>GMKGENMMVKLIALYEQPEDKQAFDEHYFNTHAPLTRK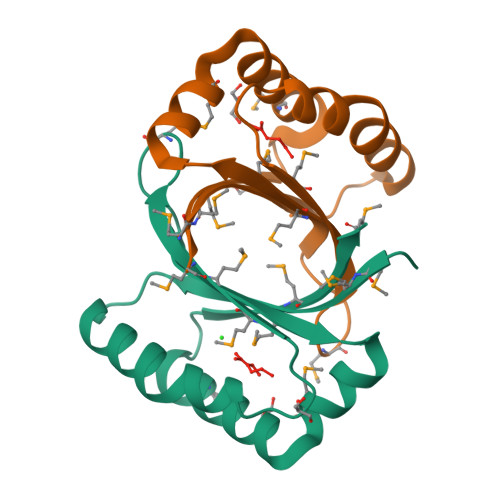IPGLRDMKVTRIVGSPMGESKFYLMCEMYYDDHESLQQAMRTDEGKASGKDAMKFAGKLLTLMIGEEMDE[2x]(2R,5R)-2-[(R)-carboxy{[(2R)-2-{[(4-ethyl-2,3-dioxopiperazin-1-yl)carbonyl]amino}-2-(4-hydroxyphenyl)acetyl]amino}methyl]-5-methyl-5,6-dihydro-2H-1,3-thiazine-4-carboxylic 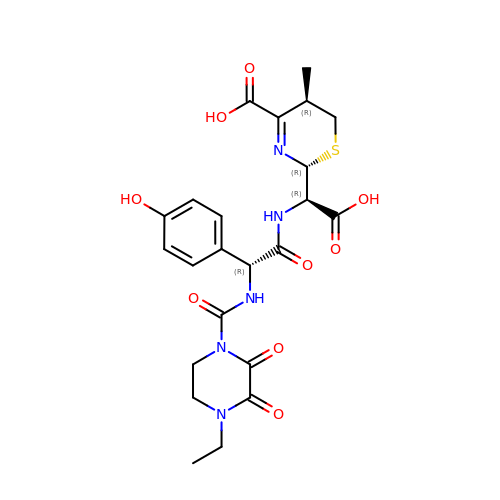acid | C23 H27 N5 O9 S | YNTRKCUUJNUMAH-QOQPWIFLSA-N> MNTEIISPHHYVYPNTTTLKNKYGIKNLNAFLEKCSHDTAKAMINLREESLPEYFDTAYLCHIHQQLFKNTFEWAGYLRHIPFTFADGTTAAMPEMKRTGWKNAFAIGDEIQEGLQRLDQTLAEKNNLQGLTREEFNSEAIELFNSLNQLHPFREGNGRTQRLFFENLAKAAGHQLNFSLITKERMMVASVAVAENGDLEPMQHLFEDISNPEKIRLLKEFMHTMKNTGRNVNDRPVMVAKEGETYTGTYRGAGLEGFALNVKGAYIIGNIDHLPPEQLKILKPGDKITFTAPKAH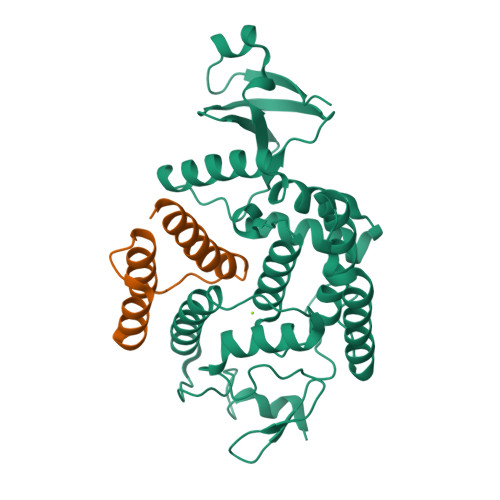HHHHH;> MVTVEATENLLSITLEELKKRREAVDAVISTHALEGIALHPKTLKILEGYARGNTSLEEFNTLMDNAKL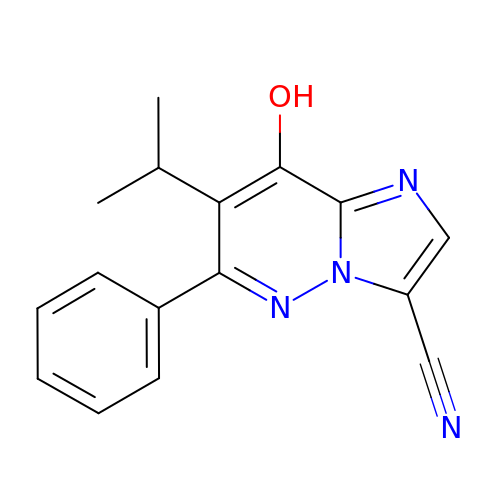8-oxidanyl-6-phenyl-7-propan-2-yl-imidazo[1,2-b]pyridazine-3-carbonitrile | C16 H14 N4 O | WZFZMEFQZHKQIH-UHFFFAOYSA-N Integrin α6β4 is a major component of hemidesmosomes that mediate the stable anchorage of epithelial cells to the underlying basement membrane. The β4 subunit only pairs with the α6 subunit to form the α6β4 integrin, which is a laminin receptor required for maintaining the integrity of epithelia. The third and fourth fibronectin type III domains (FnIII-3,4) of integrin β4 mediate binding to the hemidesmosomal proteins BPAG1e and BPAG2, and participate in signalling. The crystal structures of the individual FnIII-3 and FnIII-4 domains were solved and the relative arrangement of the FnIII domains was elucidated by combining DEER with site-directed spin labelling.

The structure of FnIII-3 (1457–1548) was refined against data to 1.60 Å resolution. The asymmetric unit contains two copies of FnIII-3 that are almost identical. After superimposition, the root-mean-square difference (r.m.s.d.) for all main-chain atoms between the two molecules is 0.59 Å. In our crystal structure β-strand A extends to A1468, similarly to as observed in other FnIII domains. Y1494 and Y1526 in FnIII-3, which are phosphorylated during signalling, are adjacent in the structure. Near Y1526, one of the FnIII-3 molecules has a sulfate ion coordinated by E1501, H1503 and two of the waters in the cleft. This anion is of interest because sulfates frequently mimic the phosphate group of phosphorylated residues. In the other FnIII-3 molecule in the asymmetric unit the position of the sulfate is occupied by the carboxylate of D1519 from a neighbouring molecule in the crystal. Collectively, the pocket near Y1526 has a propensity to bind negatively charged groups, despite being surrounded by the acidic residues E1501, E1518 and D1519. The sulfate near Y1526 in the crystal structure suggests that FnIII-3 might tolerate phosphorylation at this position.

>GSHMVPDTPTRLVFSALGPTSLRVSWQEPRCERPLQGYSVEYQLLNGGELHRLNIPNPAQTSVVVEDLLPNHSYVFRVRAQSQEGWGREREGVITI[2x]> MKFVHPRHWILQWKIRPGDKVVVISGKFKTIRGTVLQIDKMRNGVSVSGVKEQKRVKQEDGSFIRIPGLIHVSNVMLIDQAIDLPTRV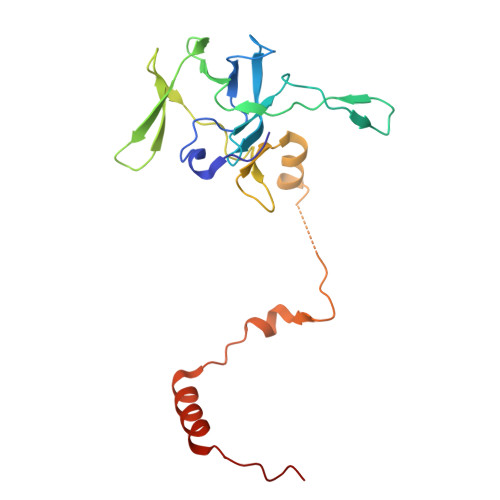ALRVDDRGNVVRISKKSGLVIPWPNGEMIKFGDNRKSREFLKSKEERDVELRKEQNDDEERAGPKDTPAEVAVERTYDYQRDVATMQALRQMMTKYNRDFR>[2x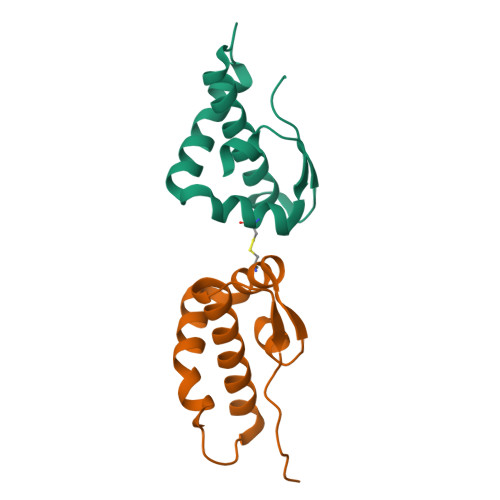]GPLGSTFEEMALTTFMITKESYCKLKNSVSDVAFNRYLSLYNKYRYFSGKMDTAAYREAACSQLAKAMETFNHNNGNDVLYQPPTASVTTSFLQ>GSHMSHLDNTMAIRLLPLPVR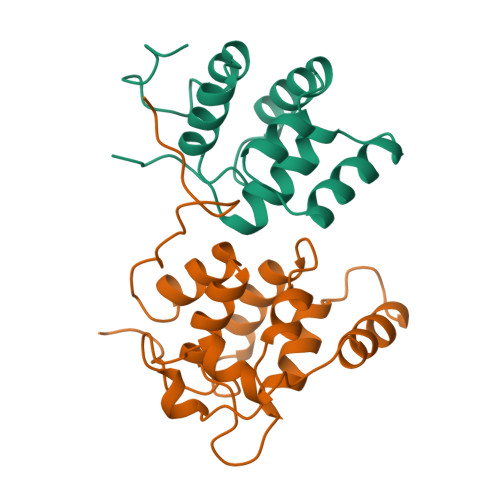AQLCAHLDALDVWQQLATAVKLYPDQVEQISSQKQRGRSASNEFLNIWGGQYNHTVQTLFALFKKLKLHNAMRLIKDYVSEDLHKYI[2x];>[2x]LSSKYSRNTELRRVEDNDIYRLAKILDENSCWRKLMSIIPKGMDVQACSGAGCLNFPAEIKKGFKYTAQDVFQIDEAANRLPPDQSKSQMMIDEWKTSGKLNERPTVGVLLQLLVQAELFSAADFVALDFLNESTPARPVDGPGALISLELLE>[2x]MEQEKVQELVSQMTLDEKIAQCLQLSPFLFKGTNKNAELTGPLLQEMKLTDAHTENAGSVLGSSSALDMIGIQEAYLKTNRLGIPLVFMADVIHGYKTVFPIPLALGCSFDRETVRVMAEVSALEATADGHHVTFSPMLDLVRDPRWGRVMESTGEDPFLNSELGKAMVDGYQGDASKLNENLEQMAACVKHFAAYGAAEAGLEYNTVNMSTRELYQNYLPAYNAAIQAGAKLVMTAFNVVDGIPATMNKWLNRDVLRGEMEFDGVLISDWGAVAEVINHGTARNPKEAAQFSMEAGVDLEMMTTCYIHELKGLIEEGKLSENLLDEAVLRMLNLKNDLGLFEDPYRGLKNNDRTKDILTDESRGKARAAGVESAVLLENKSRLLPLA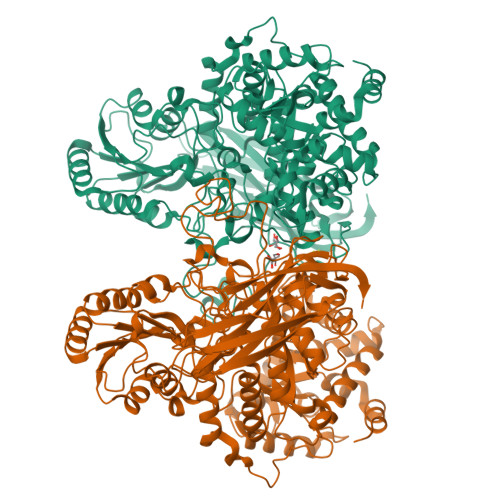KEAKIALVGPLATSPDILGGWNVYGEEKDGINVETGLREVFETVEVVSTEYTELSEEDKVAVKAAVQNMDVVVLALGEKNEWGGEAGSLATIRLPEAQYQLAKFVQTLGKPVVITLFNGRPLEVKELAESSDALLELWFPGTEAGRVTADLLSGASNPSGKLSMSFPQTTGQIPVYYNHLRTGRPQTPENKGERYVSHYLDIPNEPFYPFGYGKSYSEFELKTSSLPKELNLGESLHVEVTIKNISDIAGKEVIQVYLQDVTASISRPVKELKAFEKVALQAGEEKTVTFELTSEAFSFYNHQLEKVQEPGLHRVFVGTSSEDVDVFEVEVGGYVLEHHHHHH>GGCGAGGAACCGGGGAGCC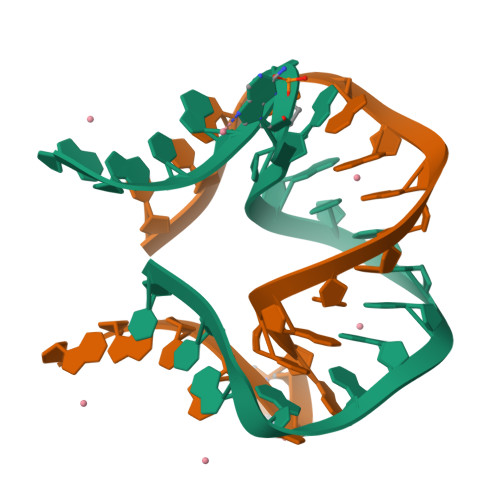[2x]> GMTKKTGFFKRLKALTLPQKQLFATALCQRMLPNYQLFSEVCEFGDPAVLSTALELLWQS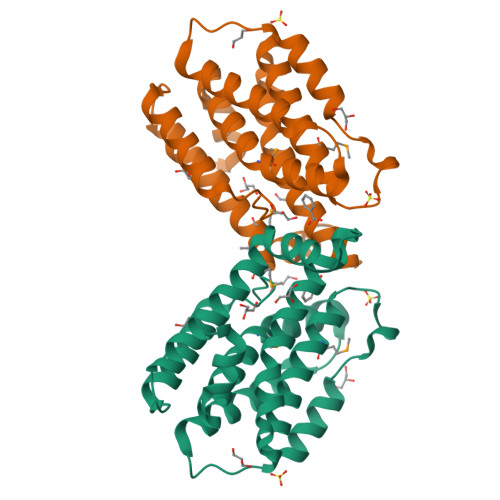LYDPKLKFNIDVHLQRLEDNTPEPADFEAYGVYPAMDAVVAISTLLGAIQGKIEEDIVNISKLSSSTVANYIEAISDVDLVDEALDDFVFAHEVMEEEKELQNSLLEIIEENPKITAELVKGLRKDIIETGVSNIGISVA>GSHMGDLKYSLERLREILERLEENPSEKQIVEAIRAIVENNAQIVEAIRAIVENNAQIVENNRAIIEALEAIGVDQKILEEMKKQLKDLK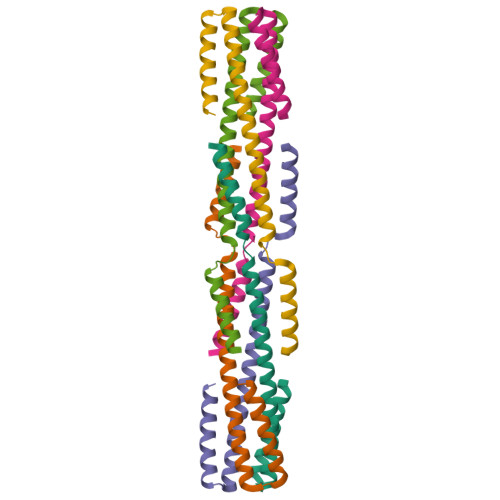RSLERG[3x]>MPRGSRSRTSRMAPPASRAPQMRAAPRPAPVAQPPAAAPPSAVGSSAAAPRQPGLMAQMAITAAGVAVGSAVGHTLGHAITGGFSGGSNAEPAR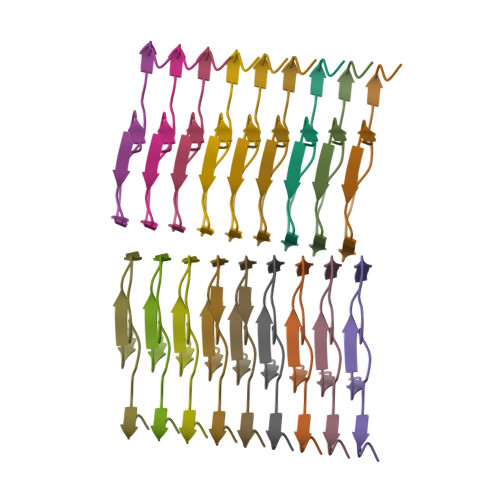PDITYQEPQGTQPAQQQQPM[18x]> GMDDLSEFVDQVPLLDHHCHFLIDGKVPNRDDRLAQVSTEADKDYPLADTKNRLAYHGFLALAKEFALDANNPLAAMNDPGYATYNHRIFGHFHFKELLIDTGFVPDDPILDLDQTAELVGIPVKAIYRLETHAEDFMLEHDNFAAWWQAFSNDVKQAKAHGFVGFKSIAAYRVGLHLEPVNVIEAAAGFDTWKHSGEKRLTSKPLIDYMLYHVAPFIIAQDMPLQFHVGYGDADTDMYLGNPLLMRDYLKAFTK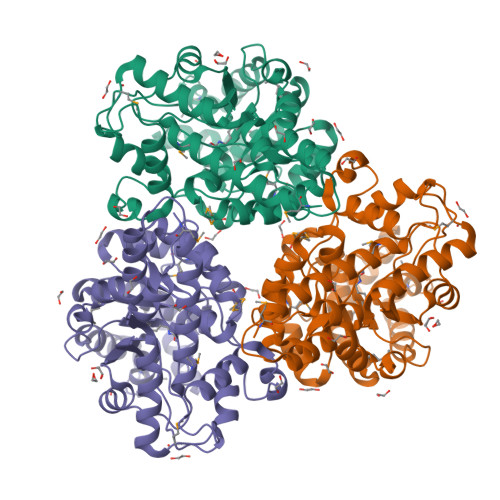KGLKVVLLHCYPYHREAGYLASVFPNLYFDISLLDNLGPSGASRVFNEAVELAPYTRILFASDASTYPEMYGLAARQFKQALVAHFNQLPFVDLAQKKAWINAICWQTSAKLYHQERELRV In this study, we present the crystallization and structure determination of a GH3 β-glucosidase from N. crassa (NcCel3A) solved to 2.25 Å resolution. The overall structure of NcCel3A is composed of three separate domains connected by two linkers and has a high degree of N-glycosylation. The two NcCel3A protein chains form a dimer similar to those observed in ReCel3A and AaBGL1. The structural analysis further showed that NcCel3A should have a similar substrate specificity to the previously structurally and biochemically characterized ReCel3A.

The final NcCel3A structure is composed of two noncrystallographic symmetry (NCS)-related molecules with 842 and 843 amino-acid residues, respectively, 875 water molecules and 85 carbohydrate residues. There are 15 NXT/S N-glycosylation sites in NcCel3A and all are found on or near the surface of the protein molecule. The majority of the long N-glycan chains are positioned on domain 1 and domain 2, and are also asymmetrically distributed onto the same face of the protein. Domain 1 of NcCel3A contains the catalytic nucleophile Asp276, as well as the majority of residues comprising substrate-binding subsite −1, with the catalytic centre being located between subsites −1 and +1. Loop IV is a 23-residue loop in which the catalytic acid/base Glu505 is located. The loss of overall protein stability owing to the lack of central secondary elements may be mitigated by the introduction of a disulfide bridge between the two strands (Cys69 and Cys85 in NcCel3A). The extended loop V, which was first observed in the structures of AaBGLI and ReCel3A, encompasses domain 1 and interacts with loop II on the opposite side of the molecule from domain 3. Loop V folds over three large N-glycan chains (bound to Asn61, Asn311 and Asn318). No distinct density corresponding to a bound glucose was observed in subsite −1 of NcCel3A, in contrast to several other GH family 3 structures. Thus, similar to ReCel3A the existence of a +2 subsite is less pronounced in NcCel3A than in HjCel3A and the enzyme may also have a substrate specificity similar to that of ReCel3A.

>[2x]APEPIHPSHQQLNKRSLAYSEPHYPSPWMDPKAIGWEEAYEKAKAFVSQLTLLEKVNLTTGIGWGAEQCVGQTGAIPRLGLKSMCMQDAPLAIRGTDYNSVFPAGVTTAATFDRGLMYKRGYALGQEAKGKGVTVLLGPVAGPLGRAPEGGRNWEGFSTDPVLTGIAMAETIKGTQDAGVVACAKHFIGNEQEHFRQVGESQDYGYNISETLSSNIDDKTMHEMYLWPFVDAIRAGVGSFMCAYTQANNSYSCQNSKLLNNLLKQENGFQGFVMSDWQAHHSGVASAAAGLDMSMPGDTMFNSGRSYWGTNLTLAVLNGTVPQWRIDDMAMRIMAAFFKVGQTVEDQEPINFSFWTLDTYGPLHWAARKDYQQINWHVNVQGDHGSLIREIAARGTVLLKNTGSLPLKKPKFLAVIGEDAGPNPLGPNGCADNRCNNGTLGIGWGSGTGNFPYLVTPDQALQARAVQDGSRYESVLRNHAPTEIKALVSQQDATAIVFVNANSGEGFIEIDGNKGDRLNLTLWNEGDALVKNVSSWCNNTIVVLHTPGPVLLTEWYDNPNITAILWAGMPGQESGNSITDVLYGRVNPSGRTPFTWGATRESYGTDVLYEPNNGNEAPQLDYTEGVFIDYRHFDKANASVLYEFGFGLSYTTFEYSNLKIEKHQVGEYTPTTGQTEAAPTFGNFSESVEDYVFPAAEFPYVYQFIYPYLNSTDMSASSGDAQYGQTAEEFLPPKANDGSAQPLLRSSGLHHPGGNPALYDIMYTVTADITNTGKVAGDEVPQLYVSLGGPEDPKVVLRGFDRLRVEPGEKVQFKAVLTRRDVSSWDTVKQDWVITEYAKKVYVGPSSRKLDLEEVLP> MEQNLFALSLDDTSSVRGSLLDTKFAQTRVLLSKAMAGGDVLLDEYLYDVVNGQDFRATVAFLRTHVITGKIKVTATTNISDNSGCCLMLAINSGVRGKYSTDVYTICSQDSMTWNPGCKKNFSFTFNPNPCGDSWSAEMISRSRVRMTVICVSGWTLSPTTDVIAKLDWSIVNEKCEPTIYHLADCQNWLPLNRWMGKLTFPQGVTSEVRRMP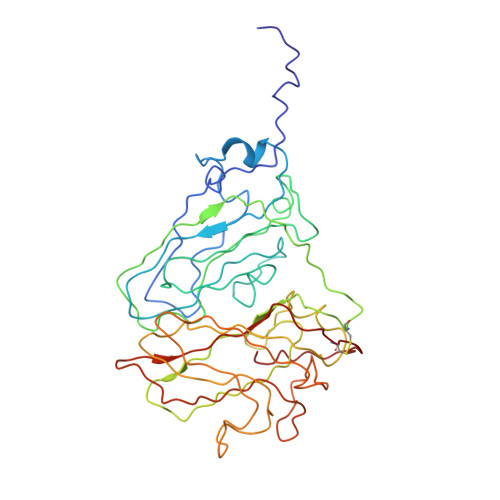LSIGGGAGATQAFLANMPNSWISMWRYFRGELHFEVTKMSSPYIKATVTFLIAFGNLSDAFGFYESFPHRIVQFAEVEEKCTLVFSQQEFVTAWSTQVNPRTTLEADGCPYLYAIIHDSTTGTISGDFNLGVKLVGIKDFCGIGSNPGIDGSRLL> LEEKKVCQGTSNKLTQLGTFEDHFLSLQRMFNNCEVVLGNLEITYVQRNYDLSFLKTIQEVAGYVLIALNTVERIPLENLQIIRGNMYYENSYALAVLSNYDANKTGLKELPMRNLQEILHGAVRFSNNPALCNVESIQWRDIVSSDFLSNMSMDFQNHLGSCQKCDPSCPNGSCWGAGEENCQKLTKIICAQQCSGRCRGKSPSDCCHNQCAAGCTGPRESDCLVCRKFRDEATCKDTCPPLMLYNPTTYQMDVNPEGKYSFGATCVKKCPRNYVVTDHGSCVRACGADSYEMEEDGVRKCKKCEGPCRKVCNGIGIGEFKDSLSINATNIKHFKNCTSISGDLHILPVAFRGDSFTHTPPLDPQELDILKTVKEITGF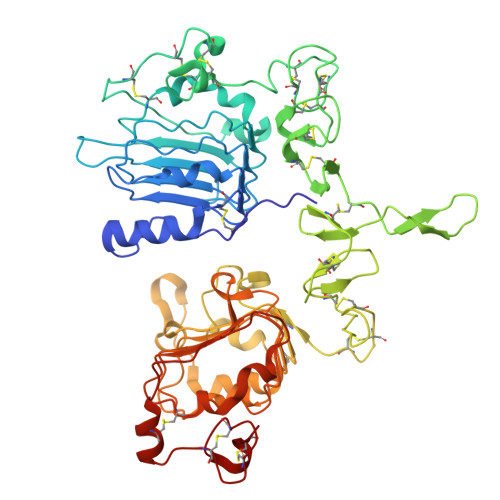LLIQAWPENRTDLHAFENLEIIRGRTKQHGQFSLAVVSLNITSLGLRSLKEISDGDVIISGNKNLCYANTINWKKLFGTSGQKTKIISNRGENSCKATGQVCHALCSPEGCWGPEPRDCVS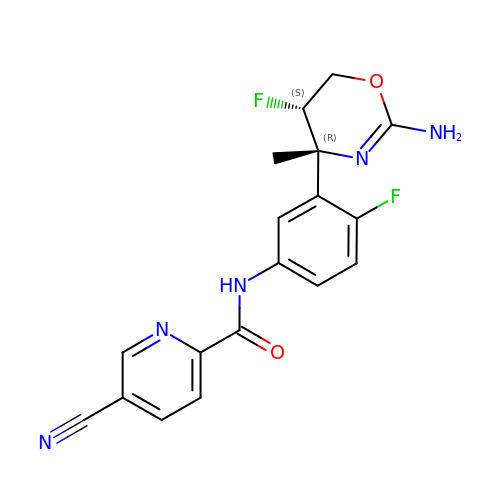N-{3-[(4R,5S)-2-amino-5-fluoro-4-methyl-5,6-dihydro-4H-1,3-oxazin-4-yl]-4-fluorophenyl}-5-cyanopyridine-2-carboxamide | C18 H15 F2 N5 O2 | ALKHFUPBQSAGMS-CRAIPNDOSA-N>[2x]MHHHHHHMETGP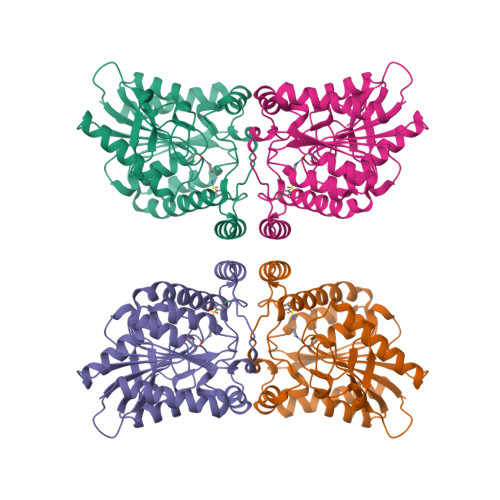EDPSSMPEESSPRRTPQSIPYQDLPHLVNADGQYLFCRYWKPTGTPKALIFVSHGAGEHSGRYEELARMLMGLDLLVFAHDHVGHGQSEGERMVVSDFHVFVRDVLQHVDSMQKDYPGLPVFLLGHSMGGAIAILTAAERPGHFAGMVLISPLVLANPESATTFKVLAAKVLNLVLPNLSLGPIDSSVLSRNKTEVDIYNSDPLICRAGLKVCFGIQLLNAVSRVERALPKLTVPFLLLQGSADRLCDSKGAYLLMELAKSQDKTLKIYEGAYHVLHKELPEVTNSVFHEINMWVSQRTATAGTASPP1-[(1S)-1-methyl-5-oxidanyl-1,2-dihydrobenzo[e]indol-3-yl]hexan-1-one 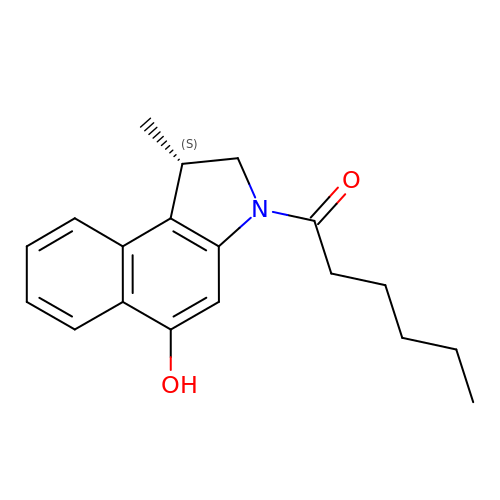| C19 H23 N O2 | RUAITRBXVQXTLB-CYBMUJFWSA-N> MGGGFAVNYNFDEIIDRRYTNAMNVEGYKGYLFGDADTSDLKDNDELIRMWVADMDFGTPEVVLNAIRERLNKKILGYTNVFGSEYYEAFVSWTKKRYGFTFSQEHLVFSHGIVAGLIELVGYICDKDDKALIVTPSYGPFKMACDKNHISTVYSPLINHHGYYEIDFDDVRKKVETENIKLCIFANPHNPTGRVWSEEELATLGQIMKENDVWLISDEIHCDIKRSGQSHIPFAKAVPDYDKIITTMSQSKAFNIAGLMFSNIIIQNESLLKTWNTHHFGTENPLSVVATQAAYEKGEGWLQAMNHYLDDNFNYLADFLEKELPHAEFKIPEATYLAWVDLSYYIKEKDIDESMAKFFIKNAGVIIEGAEQ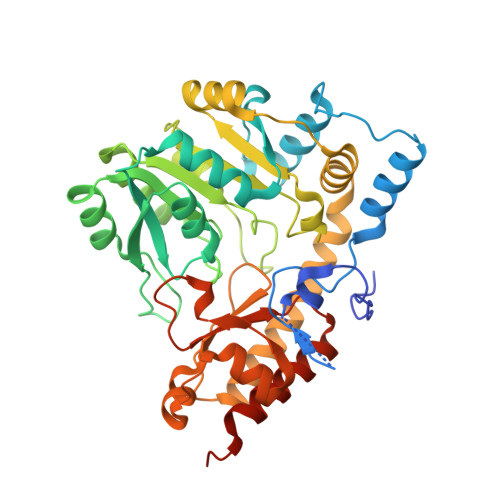FVHNAEGHIRINIAVPREVMKKGLQKIKAALVENLYFQGHHHHHHHHHH> 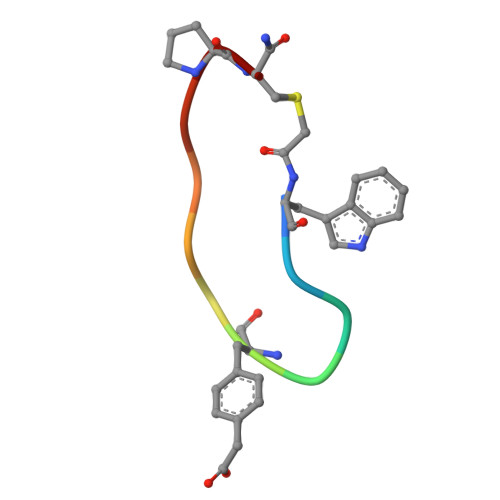WFEGFDNTFPX>SGLVPRGSHMIQQIHFYDIPRNRDEDDRTWNPNTSKTRLTLTYKRLPYKTIWVEYPDIERVCKEIGAEPSAFGLLKEGKPYYSLPVIHDPNTGTTISDSIRIARYLDKTYPDTPAVIPAELEAFHAVFEDAFWDTIFMPLFPFLVPAACPQLNPRSEAYFRETREGKFGSILGGKMENWAPTGPVRDDRWKALQAGFTKMAGWLSADGQERPFFMGEKLCYTDIV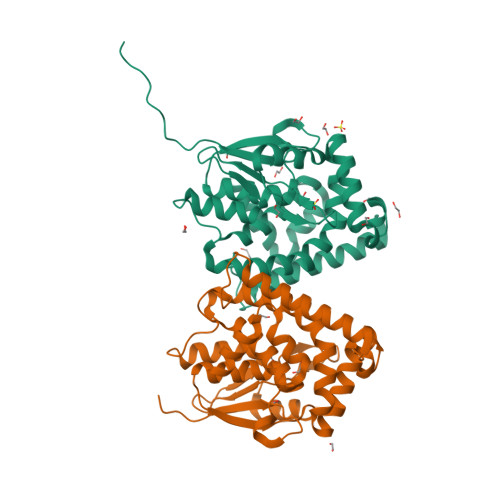VGAWLISVKKVFGSDHPEWLQVEKWDGGRWSRLVQVVENF[2x]>[4x]AMGQRAMKFCQGVVRELMSK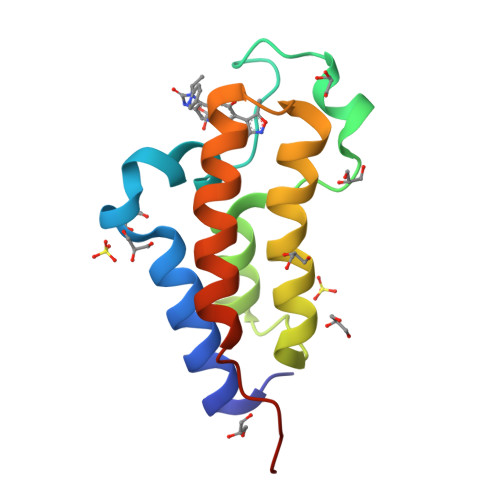KYASFNYPFLEPVDPVALNCPTYFDYVKEPMDLGTVSKKLSNWEYENLDQAEHDIRLIFQNCYAFNPDGTIVNMMGHRLEDIFNTKWADRPLYSDVES>MSTLGHQYDNSLVSNAFGFLRLPMNFQPYDSDADWVITGVPFDMATSGRAGGRHGPAAIRQVSTNLAWEHNRFPWNFDMRERLNVVDCGDLVYAFGDAREMSEKLQAHAEKLLAAGKRMLSFGGDHFVTLPLLRAHAKHFGKMALVHFDAHTDTYANGCEFDHGTMFYTAPKEGLIDPNHSVQIGIRTEFDKDNGFTVLDACQVNDRSVDDVIAQVKQIVGDMPVYLTFDIDCLDPAFAPGTGTPVIGGLTSDRAIKLVRGLKDLNIVGMDVVEVAPAYDQSEITA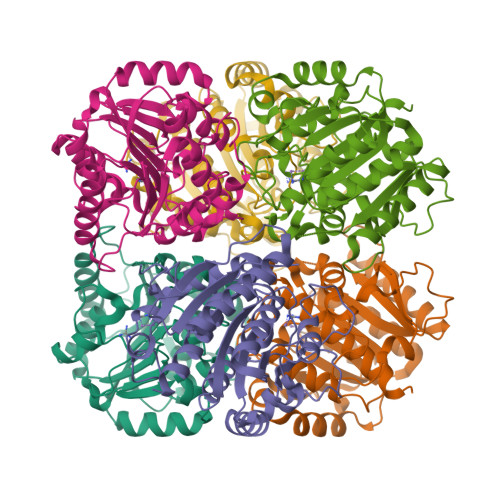LAAATLALEMLYIQAAKKGE[3x]>MVKQVFNFNAGPSALPKPALERA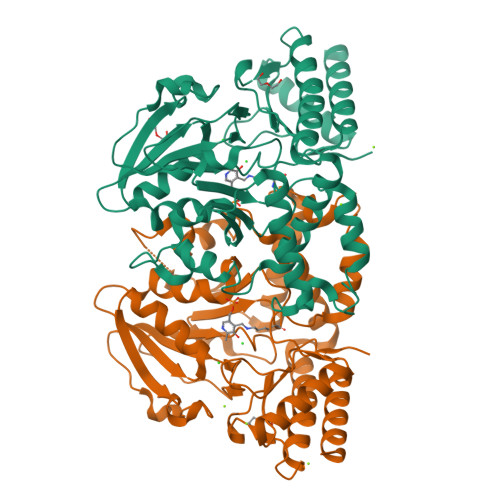QKELLNFNDTQMSVMELSHRSQSYEEVHEQAQNLLRELLQIPNDYQILFLQGGASLQFTMLPMNLLTKGTIGNYVLTGSWSEKALKEAKLLGETHIAASTKANSYQSIPDFSEFQLNENDAYLHITSNNTIYGTQYQNFPEINHAPLIADMSSDILSRPLKVNQFGMIYAGAQKNLGPSGVTVVIVKKDLLNTKVEQVPTMLQYATHIKSDSLYNTPPTFSIYMLRNVLDWIKDLGGAEAIAKQNEEKAKIIYDTIDESNGFYVGHAEKGSRSLMNVTFNLRNEELNQQFLAKAKEQGFVGLNGHRSVGGCRASIYNAVPIDACIALRELMIQFKENA[2x]> MEQKQQSERLGTEAIPKLLRSLSIPAMIGMFVMALYNVVNTIFISYAVGIEGVAGVTIAFPIMMIMMSMAGALGIGGASVISRRLGERRGEEANQVFGNILTVILVLSVIGFISAFTLLGPALQLFGATSVTQGYATDYLFPILLGSIFFFFAFAANNIIRSEGNATFAMVTMIVPAVLNILLDVLFIFGLNMGVLGASIATVIAQASVTGLVLRYFLTGKSTLSLHWSDLRMKGSVIKEVCLVGLPAFVQQSSASLMMIAINSMLLRFGSDFYVGVFGLVQRIMMFVMMPMMGIMQAMQPIV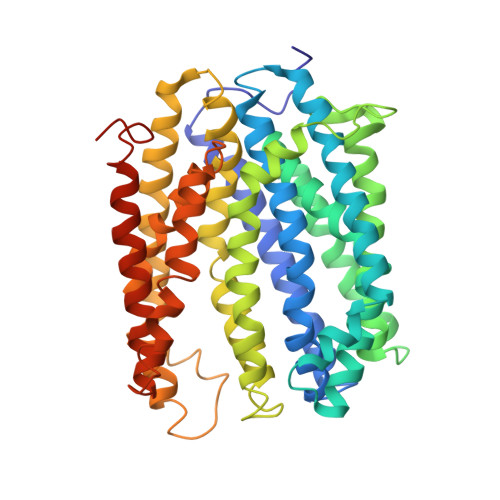GYNYGAKQYSRLRETVMLGFKVATIFSIGIFALLMLFPEALLRVFTADREVIQAGVSAMHILFCVTFLIGAQIVAGGLYQSLGKPKQALILSLSRQIIFLIPLVLILPHIFGLSGVWWAFPIADVLSFILTVVLLYRDRNVFFLKTKEERELDLVKTASS>MGSHQEYIKKVTDELKELIQNVNDDIKEVEKNPEDMEYWNKIYRLVHTMKEITETMGFSSVAKVLHTIMNLVDK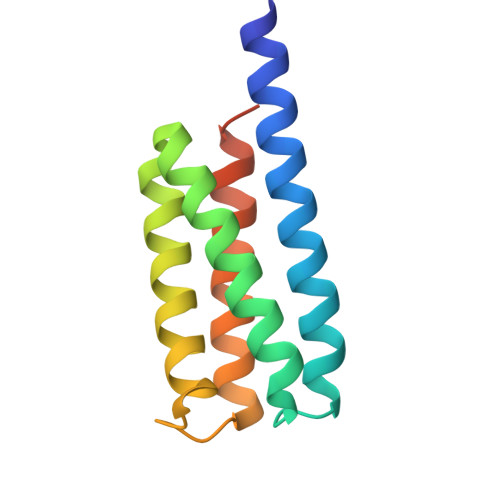MLNSEIKITSDLIDKVKKKLDMVTRELDKKVSGSYLVPR[2x]> MSLADGHHLLGNPAAKLRLVEFVSYTCPHCSHFEIESEGQLKIGMVQPGK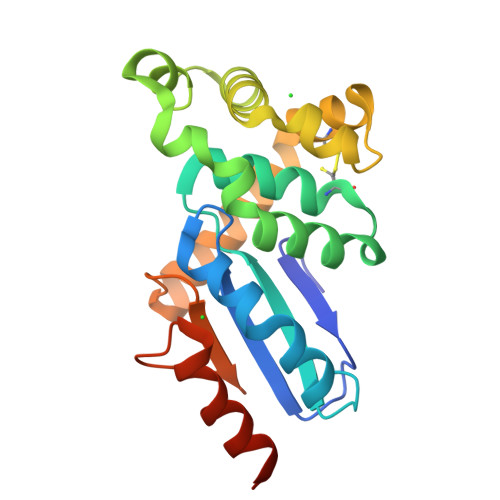GAIEVRNFVRDPIDMTVALITNCVPPSRFFTLHTAFMRSQAQWIGPLANSTEAQRQRWFNGTFATRTRAIASDFRFYDFMAARGMDRSTLDRCLSNEALAKKLAAETDEAINQYNVSGTPSFMIDGILLAGTHDWASLRPQILARLNEGHHHHHH>[4x]MRNTKRAVVFAGDYAYIR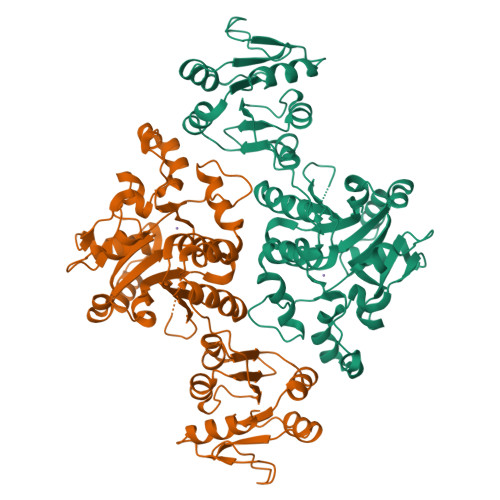QIETAMKSLCRHNSHLKIYLLNQDIPQEWFSQIRIYLQEMGGDLIDCKLIGSQFQMNWSNKLPHINHMTFARYFIPDFVTEDKVLYLDSDLIVTGDLTDLFELDLGENYLAAARSCFGAGVGFNAGVLLINNKKWGSETIRQKLIDLTEKEHENVEEGDQSILNMLFKDQYSSLEDQYNFQIGYDYGAATFKHQFIFDIPLEPLPLILHYISQDKPWNQFSVGRLREVWWEYSLMDWSVILNEWFSKSVKYPSKSQIFKLQCVNLTNSWCVEKIDYLAEQLPEVHFHIVAYTNMANELLALTRFPNVTVYPNSLPMLLEQIVIASDLYLDLNHDRKLEDAYEFVLKYKKPMIAFDNTCSENLSEISYEGIYPSSIPKKMVAAIRSYMR> K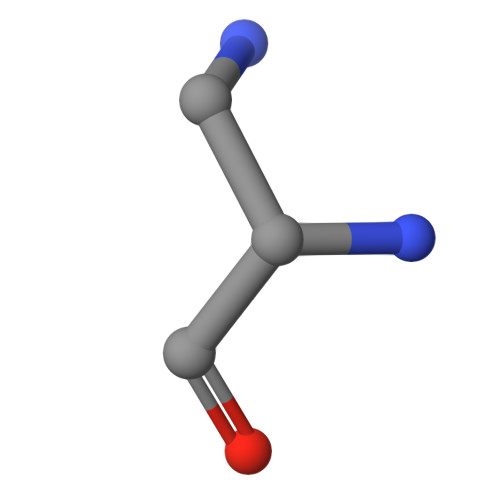AY> MASSCAVQVKLELGHRAQVRKKPTVEGFTHDWMVFVRGPEHSNIQHFVEKVVFHLHESFPRPKRVCKDPPYKVEESGYAGFILPIEVYFKNKEEPRKVRFDYDLFL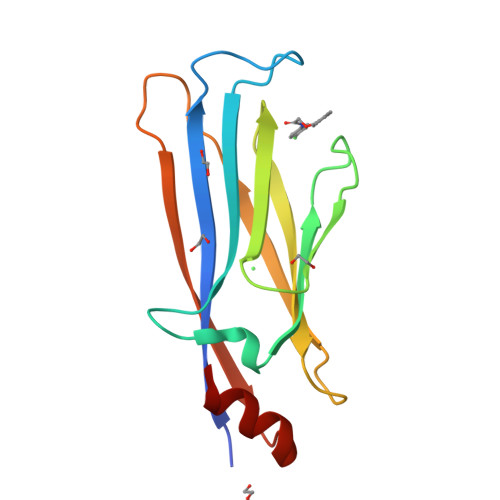HLEGHPPVNHLRCEKLTFNNPTEDFRRKLLKA> GTDERVYESIGQYGGETVKIVRIEKARDIPLGATVRNEMDSVIISRIVKGGAAEKSG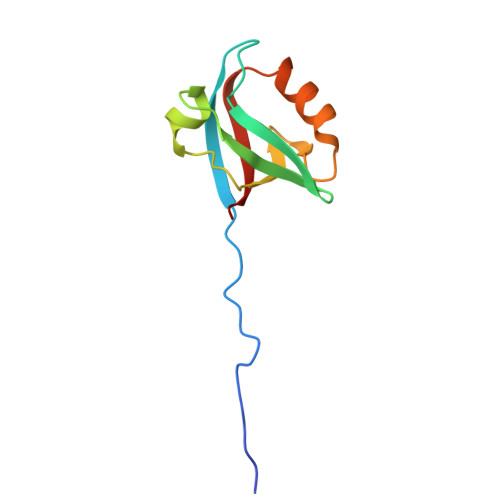LLHEGDEVLEINGIEIRGKDVNEVFDLLSDMHGTLTFVLIPSQ> GTGVPETVFEELKRYVGWGDGDERALRSLHGAAAPHFPRLAEEFYDRILGHEGARTALVGGESQVGHLKVTMIAWLDELLGGPWDEAYWDRRYRIGRVHVRIGLPQHYM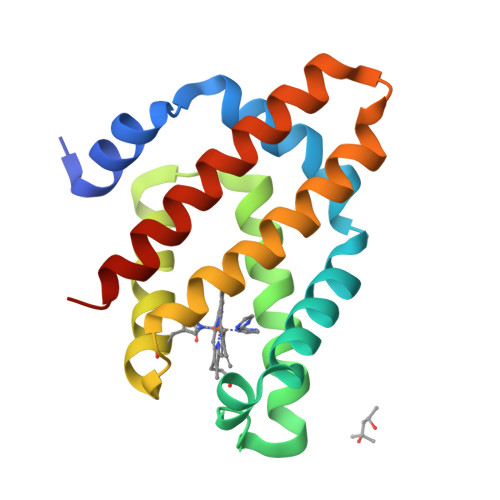FGAMNVHRTGLARLAYERFHGDPPELERVRNALGKVLDLELAVMLHTYREDL>[2x]MHHHHHHGENLYFQGSAHAMENSWTISKEYHIDEEVGFALPNPQENLPDFYNDWMFIAKHLPDLIESGQLRERVEKLNMLSIDHLTDHKSQRLARLVLGCITMAYVWGKGHGDVRKVLPRNIAVPYCQLSKKLELPPILVYADCVLANWKKKDPNKPLTYENMDVLFSFRDGDCSKGFFLVSLLVEIAAASAIKVIPTVFKAMQMQERDTLLKALLEIASCLEKA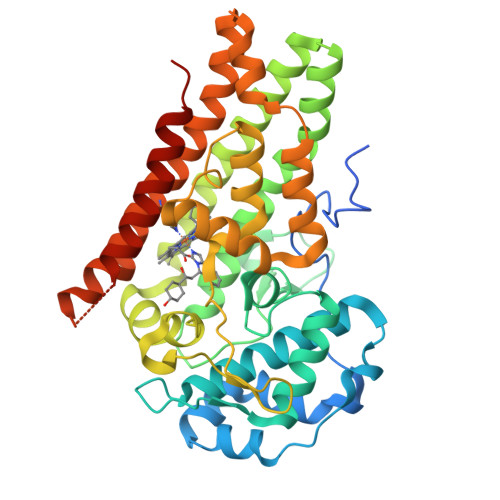LQVFHQIHDHVNPKAFFSVLRIYLSGWKGNPQLSDGLVYEGFWEDPKEFAGGSAGQSSVFQCFDVLLGIQQTAGGGHAAQFLQDMRRYMPPAHRNFLCSLESNPSVREFVLSKGDAGLREAYDACVKALVSLRSYHLQIVTKYILIPASQQPKENKTSEDPSKLEAKGTGGTDLMNFLKTVRSTTEKSLLKEGNS RECQ helicases catalyse the unwinding of duplex DNA with 3’ to 5’ directionality, driven by energy liberated by ATP-hydrolysis. RECQ-helicases are strongly implicated in the maintenance of genomic integrity, principally through their participation in the homologous recombination (HR) pathway for repair of DNA double-strand breaks and restart of collapsed or blocked replication forks, but also have roles in toleration of microsatellite instability and sister chromatid decatenation. Loss of function of WRN underlies the complex progeria Werner Syndrome; defects in BLM underlie Bloom Syndrome, which is characterised by growth retardation and immunodeficiency; and defects in RECQ4 are associated with Rothmund-Thompson syndrome, which displays growth retardation, skeletal abnormalities and premature ageing. We created the expression construct BLM-HDΔWHD to remove the conformationally flexible Winged Helix domain (WH) that requires the presence of either a stabilising nanobody, or interaction with a large DNA substrate to facilitate crystallogenesis replacing it with a short poly-(glycine/serine) linker that serves to connect the Zinc-binding domain (Zinc) directly to the Helicase and RNAse C-terminal domain (HRDC).

The aromatic-rich loop (ARL) is a highly conserved motif in RecQ helicases that serves as a molecular ‘sensor’, detecting binding of single-stranded DNA and coupling it to structural rearrangements that enable ATP hydrolysis. In our high-resolution structure of BLM-HDΔWHD, the ARL is disordered and is not visible in electron-density maps. In their paper describing the crystal structure of BLM in complex with DNA, Newman et al. observe that the HRDC domain packs against a shallow cleft formed between the D1 and D2 domains of the helicase core, with the interface between the different modules being highly polar in nature. In our high-resolution crystal structure of BLM-HDΔWHD, we observe the same ‘parked’ interaction for the HRDC, even in the absence of the WHD, but in our liganded structure we see that the HRDC domain swings across the face of the core helicase fold to make a series of polar interactions with the ssDNA-15mer, which is presented on the surface of the D1 domain of a second protomer within the asymmetric unit.

> MGSAWSHPQFEKSSGLEVLFQGPHMSRNLKHERFQSLSFPHTKEMMKIFHKKFGLHNFRTNQLEAINAALLGEDCFILMPTGGGKSLCYQLPACVSPGVTVVISPLRSLIVDQVQKLTSLDIPATYLTGDKTDSEATNIYLQLSKKDPIIKLLYVTPEKICASNRLISTLENLYERKLLARFVIDEAHCVSQWGHDFRQDYKRMNMLRQKFPSVPVMALTATANPRVQKDILTQLKILRPQVFSMSFNRHNLKYYVLPKKPKKVAFDCLEWIRKHHPYDSGIIYCLSRRECDTMADTLQRDGLAALAYHAGLSDSARDEVQQKWINQDGCQVICATIAFGMGIDKPDVRFVIHASLPKSVEGYYQESGRAGRDGEISHCLLFYTYHDVTRLKRLIMMEKDGNHHTRETHFNNLYSMVHYCENITECRRIQLLAYFGENGFNPDFCKKHPDVSCDNCCKTKGSGGSKALVAKVSQREEMVKKCLGELTEVCKSLGKVFGVHYFNIFNTVTLKKLAESLSSDPEVLLQIDGVTEDKLEKYGAEVISVLQKYSEWTSPAEDSSPG>[3x]ARKKGKSASQVIVLKEKSRKKRQKS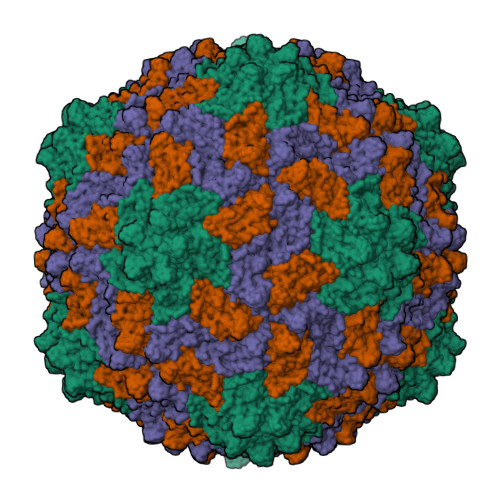RGQQPTRQVTPVSAPAAMGTQITYRGPQVVTQYGDITPAKNSGSLVRVTSSATAGTEVSGTVLFNVRNATELPWLSGQGSRYSKYRVRYAHFTWEPIVGSNTNGEVAMAMLYDVADVTSITIERLMQTRGGTWGPIWSPTRKRLSYDPEHASLPWYLSGVSSGAAAGNIQTPFQIAWAAQSSLVSTTLGRIMAEYLVELTDPVDVTINQ> GHMLDCKAVALKWVHQFRIPGGDNCNFYCSYDSLYQQFNLWKKNDACQGADGFSTAIPKIQEAPCSDCPGS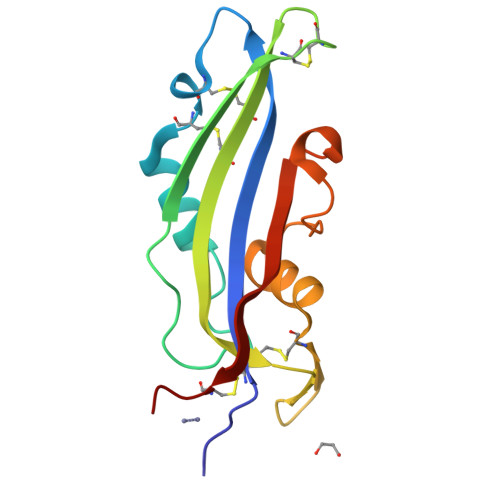KTCICSVQATAWRVRNGKWFDGQQWFDCDVKPYTERVLGRRWYDESEADKDIYVGYYSRGFISNDNVHCGSQ>VEYKNTICPPRQDYRYWYFVAELTIGVNYDINSTIIGECHMSESYIDRNANIVLTGYGLKINMTIMDTDQRFVAAAEGVGKDNKLSVLLFTTQRLDKVHHNISVTITCMEMNCGTTKYNSDLPESIHKSSSCDITINGSCVTCVNLETDPTKINPHYLHPKNKYLYHNSEYSMRGSYGVTFIDELNQCLLDIKELSYDICYRE[6x];>VIHVTKEVKEVATLSCGHNVSVEELAQTRIYWQKEKKMVLTMMSGDMNIWPEYKNRTIFDITNNLSIVILALRPSDEGTYECVVLKYEKDAFKREHLAEVTLSVKADFPTPSISDFEIPTSNIRRIICSTSGGFPEPHLSWLENGEELNAINTTVSQDPETE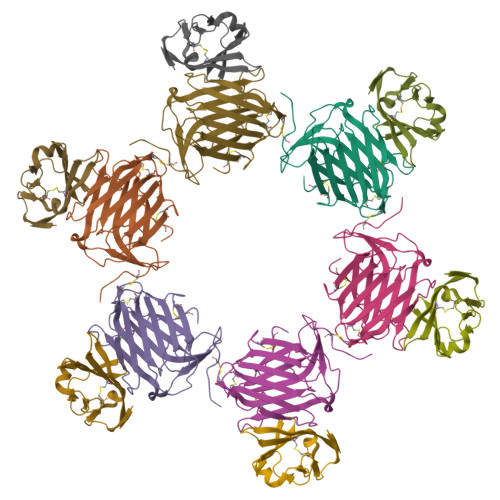LYAVSSKLDFNMTTNHSFMCLIKYGHLRVNQTFNWNTT[6x]>MQKPVCLVVAMTPKRGIGINNGLPWPHLTTDFKHFSRVTKTTPEEASRLNGWLPRKFAKTGDSGLPSPSVGKRFNAVVMGRKTWESMPRKFRPLVDRLNIVVSSSLKEEDIAAEKPQAEGQQRVRVCASLPAALSLLEEEYKDSVDQIFVVGGAGLYEAALSLGVASHLYITRVAREFPCDVFFPAFPGDDILSNKSTAAQAAAPAESVFVPFCPELGREKDNEATYRPIFISKTFSDNGVPYDFVVLEKRRKTDDAATAEPSNAMSSLTSTRETTPVHGLQAPSSAAAIAPVLAWMDEEDRKKREQKELIRAVPHVHFRGHEEFQYLDLIADIINNGRTMDDRTGVGVISKFGCTMRYSLDQAFPLLTTKRVFWKGVLEELLWFIRGDTN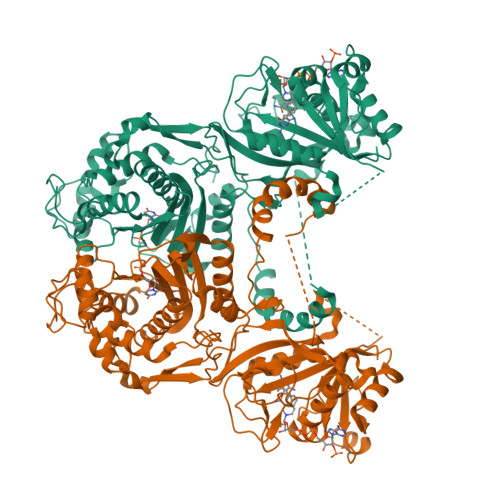ANHLSEKGVKIWDKNVTREFLDSRNLPHREVGDIGPGYGFQWRHFGAAYKDMHTDYTGQGVDQLKNVIQMLRTNPTDRRMLMTAWNPAALDEMALPPCHLLCQFYVNDQKELSCIMYQRSCDVGLGVPFNIASYSLLTLMVAHVCNLKPKEFIHFMGNTHVYTNHVEALKEQLRREPRPFPIVNILNKERIKEIDDFTAEDFEVVGYVPHGRIQMEMAV[4x]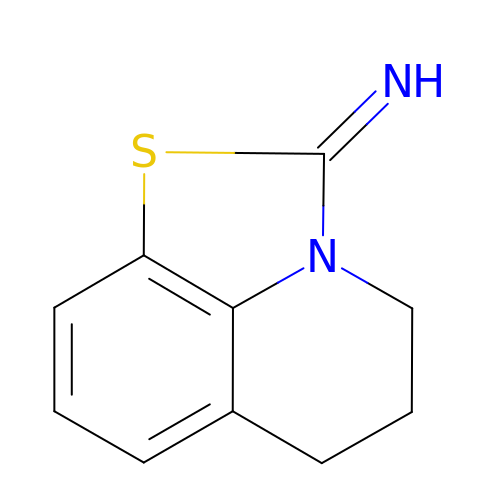5,6-dihydro-2-imino-2H,4H-thiazolo(5,4,3-IJ)quinoline | C10 H10 N2 S | JHKKLXTWYNAHPM-ZHACJKMWSA-N>[7x]AWITAPVALREGEDLSKKNPIAKIHSDLAEERGLKITYKYTGKGITEPPFGIFVFNKDTGELNVTSILDREETPFFLLTGYALDARGNNVEKPLELRIKVLDINDNEPVFTQDVFVGSVEELSAAHTLVMKINATDADEPNTLNSKISYRIVSLEPAYPPVFYLNKDTGEIYTTSVTLDREEHSSYTLTVEARDGNGEVTDKPVKQAQVQIRILDVNDNIPVVENKVLEGMVEENQVNVEVTRIKVFDADEIGSDNWLANFTFASGNEGGYFHIETDAQTNEGIVTLIKEVDYEEMKNLDFSVIVANKAAFHKSIRSKYKPTPIPIKVKVKNVKEGIHFKSSVISIYVSESMDRSSKGQIIGNFQAFDEDTGLPAHARYVKLEDRDNWISVDSVTSEIKLAKLPDFESRYVQN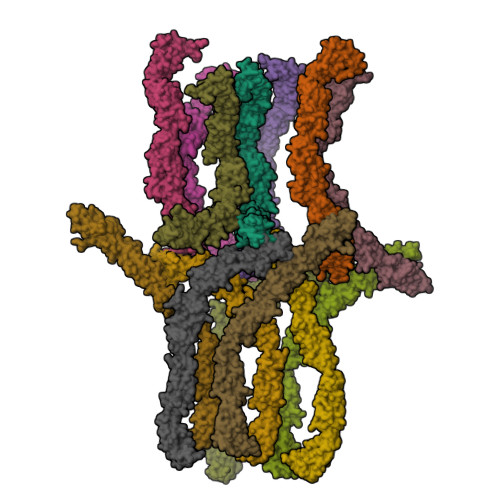GTYTVKIVAISEDYPRKTITGTVLINVEDINDNCPTLIEPVQTICHDAEYVNVTAEDLDGHPNSGPFSFSVIDKPPGMAEKWKIARQESTSVLLQQSEKKLGRSEIQFLISDNQGFSCPEKQVLTLTVCECLHGSGCREAH;>RWAPIPCSMLENSLGPFPLFLQQVQSDTAQNYTIYYSIRGPGVDQEPRNLFYVERDTGNLYCTRPVDREQYESFEIIAFATTPDGYTPELPLPLIIKIEDENDNYPIFTEETYTFTIFENCRVGTTVGQVCATDKDEPDTMHTRLKYSIIGQVPPSPTLFSMHPTTGVITTTSSQLDRELIDKYQLKIKVQDMDGQYFGLQTTSTCIINIDDVNDHLPTFTRTSYVTSVEENTVDVEILRVTVEDKDLVNTANWRANYTILKGNENGNFKIVTDAKTNEGVLCVVKPLNYEEKQQMILQIGVVNEAPFSREASPRSAMSTATVTVNVEDQDEGPECNPPIQTVRMKENAEVGTTSNGYKAYDPETRSSSGIRYKKLTDPTGWVTIDENTGSIKVFRSLDREAETIKNGIYNITVLASDQGGRTCTGTLGIILQDVNDNSPFIPKKTVIICKPTMSSAEIVAVDPDEPIHGPPFDFSLESSTSEVQRMWRLKAINDTAARLSYQNDPPFGSYVVPITVRDRLGMSSVTSLDVTLCDCITENDCTH[7x]> GSAAAPLSPAWMPAYACQRPTPLTHHNTGLSEALEILAEAAGFEGSEGRLLTFCRAASVLKALPSPVTTLSQLQG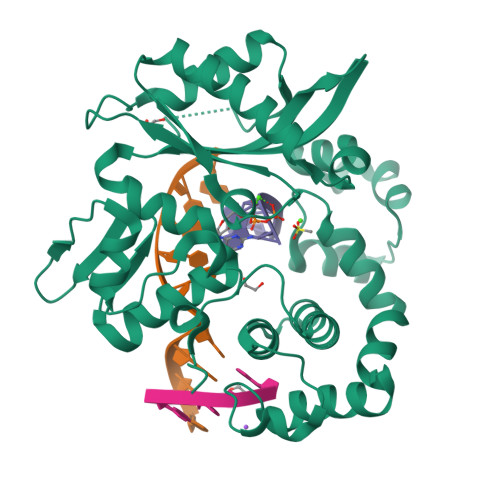LPHFGEHSSRVVQELLEHGVCEEVERVRRSERYQTMKLFTQIFGVGVKTADRWYREGLRTLDDLREQPQKLTQQQKAGLQHHQDLSTPVLRSDVDALQQVVEEAVGQALPGATVTLTGGFRRGKLQGHDVDFLITHPKEGQEAGLLPRVMCRLQDQGLILYHQHQHSCCESPTRLAQQSHMDAFERSFCIFRLPQPGSWKAVRVDLVVAPVSQFPFALLGWTGSDLFQRELRRFSRKEKGLWLNSHGLFDPEQKTFFQAASEEDIFRHLGLEYLPPEQRNA>IQTTAPPVKESSFVEKMKKTGRNIIVFYGSQTGTAEEFANRLSKDAHRYGMRGMSADPEEYDLADLSSLPEIDKSLVVFAMATYGEGDPTDNAQDFYDWLQETDVDLTGVKFAVFGLGNKCYEHFNAMGKYVDQRLEQLGAQRIFELGLGDDDGNLEEDFITWREQFWPAVAEFFGVEATGEESSIRQYELVVHEDMDVAKVYTGEMGRLKSYENQKPPFDAKNPFLAAVTANRKLNQGTERHLMHLELDISDSKIRYESGDHVAVYPANDSALVNQIGEILGADLDVIMSLNNLDEESNKKHPFPTPTTYRTALTYYLDITNPPRTNVLYELAQYASEPSEQEHLHKMASSSGEGKELYLSWVVEARRHILAILQDYPSLRPPIDHLLELLPRLQARYYSIASSSKVHPNSV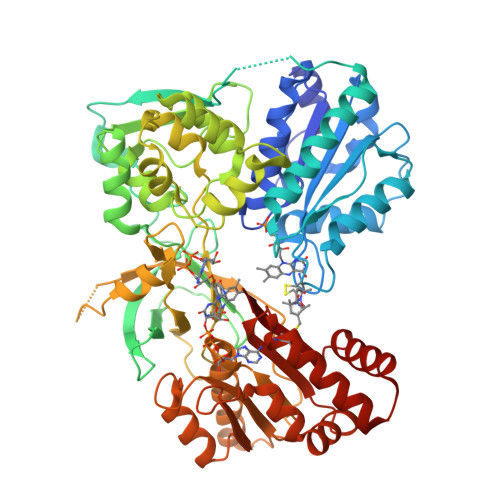HITAVAVEYEAKSGRVNKGVATSWLRAKEPAGENGGRALVPMFVRKSQFRLPFKSTTPVIMVGPGTGIAPFMGFIQERAWLREQGKEVGETLLYYGARRSDEDYLYREELARFHKDGALTQLNVAFSREQAHKVYVQHLLKRDREHLWKLIHEGGAHIYVAGDARNMCKDVQNTFYDIVAEFGPMEHTQAVDYVKKLMTKGRYSLDVWS[2x]>CGCAATTGCG[2x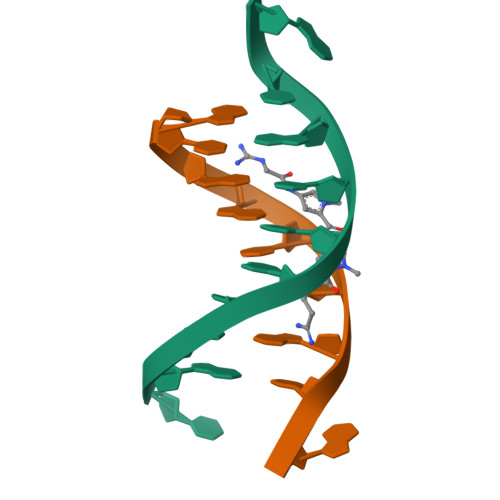]>[4x]DKNIIIGAMTALITPFKNGKVDEQSYARLIKRQIENGIDAVVPVGTTGESATLTHEEHRTCIEIAVETCKGTKVKVLAGAGSNATHEAVGLAKFAKEHGADGILSVAPFYNKPTQQGLYEHYKAI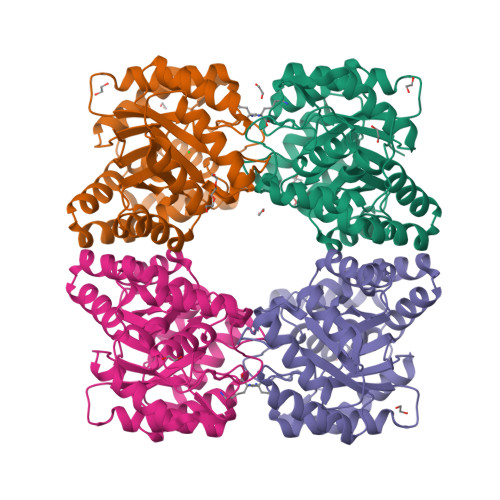AQSVDIPVLLYNVPGRTGCEISTDTIIKLFRDCENIYGVKEASGNIDKCVDLLAHEPRMMLISGEDAINYPILSNGGKGVISVTSNLLPDMISALTHFALDENYKEAKKINDELYNINKILFCESNPIPIKTAMYLAGLIESLEFRLPLCSPSKENFAKIEEVMKKYKIKGF>M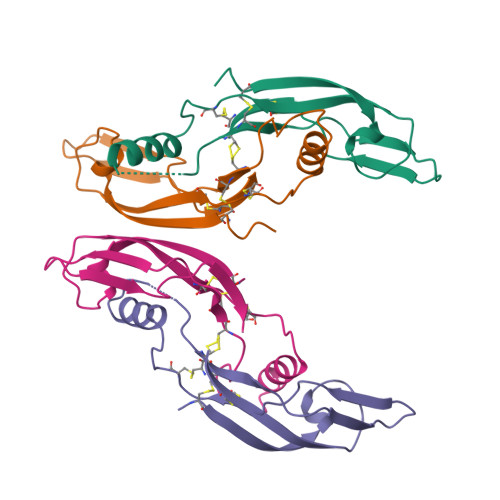SPDKQAAALPRRERNRQAAAASPENSRGKGRRGQRGKNRGCVLTAIHLNVTDLGLGYETKEELIFRYCSGSCEAAETMYDKILKNLSRSRRLTSDKVGQACCRPVAFDDDLSFLDDSLVYHILRKHSAKRCGCI[4x]>[2x]GHMGKPDISAKDLRNIMYDHLPGFGT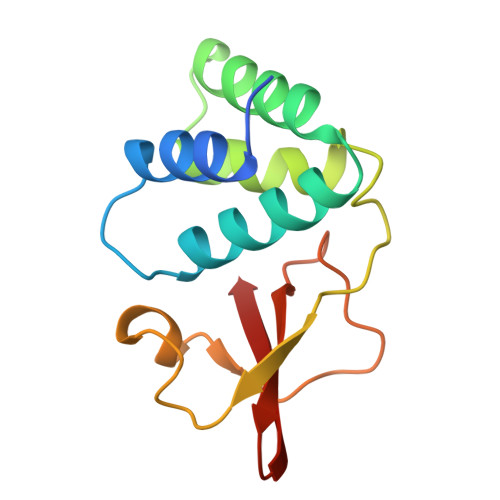AFHQLVQVICKLGKDSNSLDIIHAEFQASLAEGDSPQCALIQITKRVPIFQDAAPPVIHIRSRGDIPRACQKSLRPVPPSPKIDRGWVCVFQLQDGKTLGLKI>MTSVTSKQSTILGSDEIDLGRVIGELIDHRKLIISITSVFTLFAILYALLATPIYETDALIQIEQKQGNAILSSLSQVLPDGQPQSAPETALLQSRMILGKTIDDLNLQIQIEQKYFPVIGRGLARLMGEKPGNIDITRLYLPDSDDISNNTPSIILTVKDKENYSINSDGIQLNGVVGTLLNEKGISLLVNEIDAKPGDQFVITQLPRLKAISDLLKSFSVADLGKDTGMLTLTLTGDNPKRISHILDSISQNYLAQNIARQAAQDAKSLEFLNQQLPKVRAELDSAEDKLNAYRKQKDSVDLNMEAKSVLDQIVNVDNQLNELTFREAEVSQLYTKEHPTYKALMEKRQTLQEEKSKLNKRVSSMPSTQQEVLRLSRDVESGRAVYLQLLNRQQELNIAKSSAIGNVRIIDNAVTDPNPVRPKKTIIIVIGVVLGLIVSVVLVLFQVFLRRGIESPEQLEEIGINVYASIPISEWLTKNARQSGKVRKNQSDTLLAVGNPADLAVEAIRGLRTSLHFAMMEAKNNVLMISGASPSAGMTFISSNLAATIAITGKKVLFIDADLRKGYAHKMFGHKNDKGLSEFLSGQAAAEMIIDKVEGGGFDYIGRGQIPPNPAELLMHPRFEQLLNWASQNYDLIIIDTPPILAVTDAAIIGRYAGTCLLVARFEKNTVKEIDVSMKRFEQSGVVVKGCILNGVVKKASSYYRYGHNHYGYSYYDKKHHHHHH[8x]

Gram-negative species couple polymerization with translocation across the periplasm and outer membrane and the master regulator of the system is the tyrosine autokinase, Wzc. The tyrosine autokinase domain forms the cytoplasm region, while the periplasmic region contains small folded motifs and helical bundles. Autophosphorylation of the tyrosine-rich C-terminus of Wzc results in disassembly of the octamer into multiply phosphorylated monomers. We propose that the cycling between phosphorylated monomer and dephosphorylated octamer regulates glycan polymerization and translocation.

Previous work showed that mutation of K540 in the Walker box abrogated Wzc phosphorylation. In contrast to phosphorylated and enzymatically-dephosphorylated protein, purified non-phosphorylated WzcK540M was homogeneous, oligomeric (based on molecular mass in gel filtration) and yielded discrete octameric particles in negatively-stained EM images. A cryo-EM structure of WzcK540M at 2.85 Å resolution was determined with C1 symmetry. However, C8 symmetry breaks down for part of the periplasmic region, so local C1 refinement was used to complete the structure. In contrast to motifs 1 and 2, motif 3 (268–402) is not well ordered in the C8-averaged map and working in C1 identified three discrete structural arrangements. We designate the three possible arrangements as class i, ii and iii. In the most common particle, class i is found in three monomers (chains A, D and F) with all motif 3 residues visualised; this permits an almost complete model of the Wzc monomer. Class i is a four coiled-coil helical bundle (α8–α11), composed of two helical pairs (α8–α11 and α9–α10). Only a portion of α8 and α11 could be traced in class ii (chains B, C, G and H), where the helical axes are arranged approximately parallel to the eightfold axis. We were unable to identify any density for motif 3 in chain E (class iii).>[6x]MSIAVGMIETLGFPAVVEAADSMVKAARVTLVGYEKIGSGRVTVIVRGDVSEVQ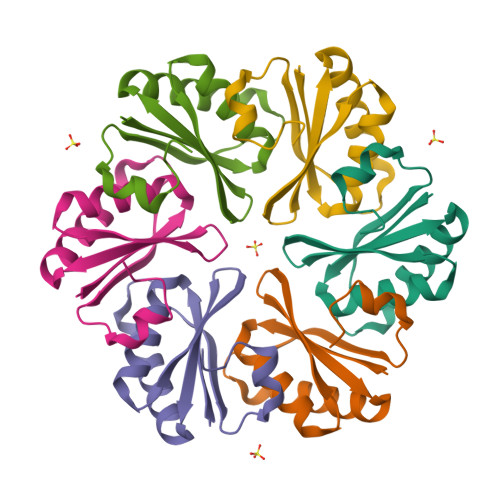ASVTAGIENIRRVNGGEVLSNHIIARPHENLEYVLPIRYTEAVEQFREIVNPSIIRRAAALEHHHHHH>GEDSLGMEVGYRLIPMVDFQQDGELLGRIRSIRKKFAQDMGFLPPVVHIRDNMDLQPARYRILMKGVEIGSGDAYPGRWLAINPGTAAGTLPGEKTVDPAFGLDAIWIESALKEQAQIQGFTVVEASTVVATHLNHLIGQFSAELFGRQEAQQLLDRVSQEMPKLTEDLVPGVVTLTTLHKVLQNLLAEKVPIRDMRTILETLAEHAPLQSDPHELTAVVRVALGRAITQQWFPGNEEVQVIGLDTALERLLLQALQGGGGLEPGLADRLLAQTQEALSRQEMLGAPPVLLVNHALRPLLSRFLRRSLPQLVVLSNLELSDNRHIRMTATIGGK[3x];>GAHMSIDETVARYKAQFTQLDTMMSKLNNTSSYLTQQFTAMNKSGGSGGSGSGGSG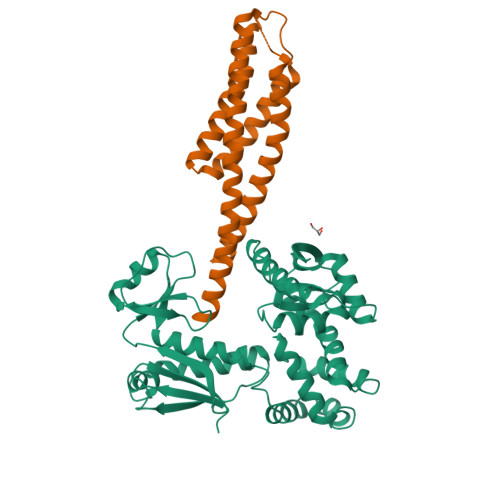GMTSTVEFINRWQRIALLSQSLLELAQRGEWDLLLQQEVSYLQSIETVMEKQTPPGITRSIQDMVAGYIKQTLDNEQLLKGLLQQRLDELSSLIGQSTRQKSLNNAYGRLSGMLLVPDAPGAS[3x]>MLNSINTNPGALLALQNLNSTNTELAATQGRINTGKKVANAKDNGAIWSMAKMQSATASSLNSVKDSLQRGQSTIDVALAAGDTITDLLTKMKEKALAASDTSLNTASFNALKADFESLRDQLQKAATNAKFNGVSLADGSTTKLSFLANEDGSNFTVTAQTLSLTGIGLTATSTFTDAATAKTMIATITTSLQTATNKLSSLGTSSVGLDTHLTFVGKLQDSLDAGVGNLVDAD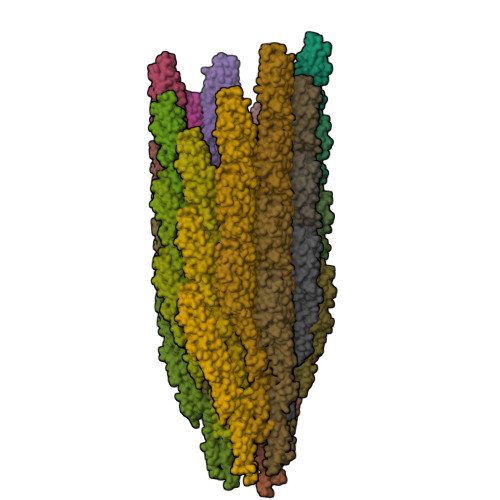LAKESAKLQSLQTKQQLGVQALSIANQTPQTILSLFKG[37x]> EQFEVIKQQKEIIEHGIELFNKKPKRGIQFLQEQGMLGTSVEDIAQFLHQEERLDSTQVGDFLGDSARFNKEVMYAYVDQLDFCEKEFVSALRTFLEGFRLPGEAQKIDRLMEKFAARYIECNQGQTLFASADTAYVLAYSIIMLTTDLHSPQVKNKMTKEQYIKMNRGINDSKDLPEEYLS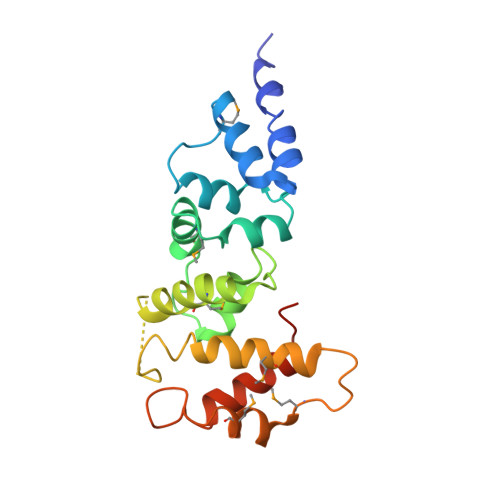SIYEEIEGKKIAMKETKELT> MASVHGTTYELLRRQGIDTVFGNPGSNELPFLKDFPEDFRYILALQEACVVGIADGYAQASRKPAFINLHSAAGTGNAMGALSNARTSHSPLIVTAGQQTRAMIGVEAGETNVDAANLPRPLVKWSYEPASAAEVPHAMSRAIHMASMAPQGPVYLSVPYDDWDKDADPQSHHLFD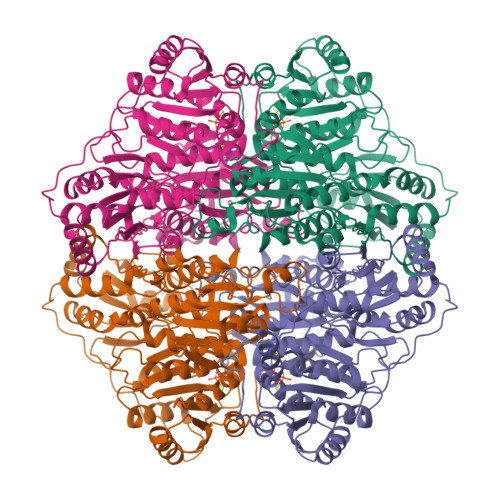RHVSSSVRLNDQDLDILVKALNSASNPAIVLGPDVDAANANADCVMLAERLKAPVWVAPSAPRCPFPTRHPCFRGLMPAGIAAISQLLEGHDVVLVIGAPVFRYHQYDPGQYLKPGTRLISVTCDPLEAARAPMGDAIVADIGAMASALANLVEESSRQLPTAAPEPAKVDQDAGRLHPETVFDTLNDMAPENAIYLNESTSTTAQMWQRLNMRNPGSYYFCAAGGLGFALPAAIGVQLAEPERQVIAVIGDGSANYSISALWTAAQYNIPTIFVIMNNGTYGMLRWFAGVLEAENVPGLDVPGIDFRALAKGYGVQALKADNLEQLKGSLQEALSAKGPVLIEVSTVSPVK> MRARRLCAAAVAAMAAASMVSACGSQTGGIVINYYTPANEEATFKAVANRCNEQLGGRFQIAQRNLPKGADDQRLQLARRLTGNDKSLDVMALDVVWTAEFAEAGWAVPLSEDPAGLAEADATENTLPGPLETARWQDELYAAPITTNTQLLWYRADLMPAPPTTWDGMLDEANRLYREGGPSWIAVQGKQYEGMVVWFNTLLQSAGGQVLSDDGQRVTLTDT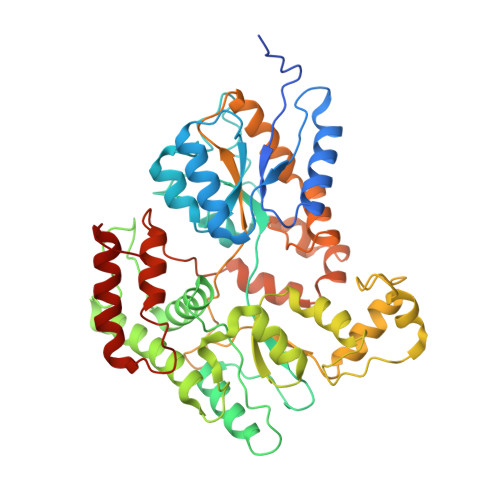PEHRAATVKALRIIKSVATAPGADPSITQTDENTARLALEQGKAALEVNWPYVLPSLLENAVKGGVSFLPLDGDPALQGSINDVGTFSPTDEQFDIAFDASKKVFGFAPYPGVNPDEPARVTLGGLNLAVASTSQHKAEAFEAIRCLRNVENQRYTSIEGGLPAVRTSLYDDPAFQKKYPQYEIIRQQLTNAAVRPATPVYQAVSTRMSATLAPISDIDPERTADELTEAVQKAIDGKGLIP> GHMRNTPAIEELDLYVWEGKADIVDRVARCMASFDVEVIRADNAAVSPERAALRRSLAIISVTMIEGGAAFLRDWQANIGMPVVWVGAARDHDASQYPPEYSHILPLDFTCAELRGMIGKLVTQLRAHAAETLQPSELVAHSESMQALLHEVDTFADCDTNVLLHGETGVGKERIAQLLHEKHSRYRHGEFVPVNCGAIPDGLFESLFFGHAKGSFTGAVVAHKGYFEQAAGGTLFLDEVGDLPLYQQVKLLRVLEDGAVLRVGATAPVKVDFRLVAASNKKLPQLVKEGLFRADLYYRLAVIELSIPSLEERGAVDKIALFKSFVAQVVGEERLAELSDLPY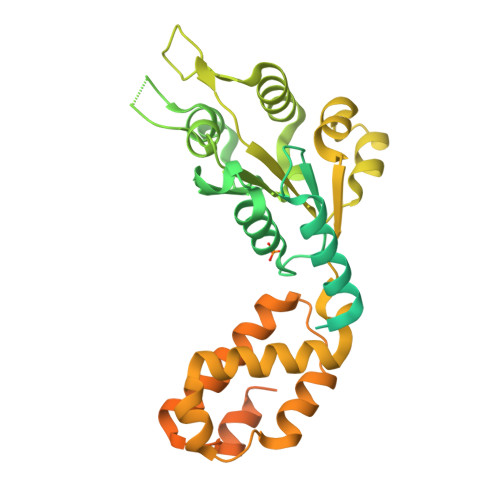WLTDSVADSYFPGNVRELRNLAERVGVTVRQTGGWDAARLQRLIAHARSAAQPVPAESAAEVFVDRSKWDMNERNRVIAALDANGWRRQDTAQQLGISRKVLWEKMRKYQIFDEEPETRESE>[4x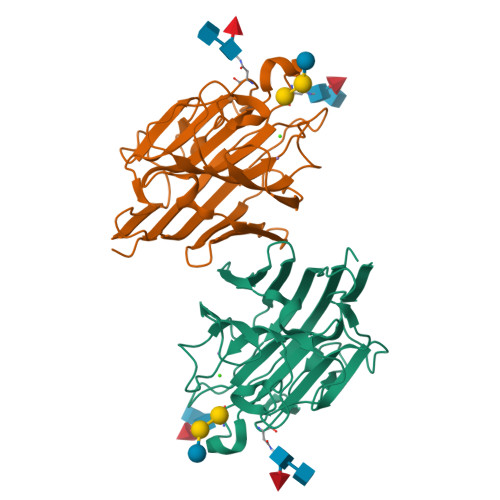]KTISFNFNQFHQNEEQLKLQRDARISSNSVLELTKVVNGVPTWNSTGRALYAKPVQVWDSTTGNVASFETRFSFSIRQPFPRPHPADGLVFFIAPPNTQTGEGGGYFGIYNPLSPYPFVAVEFDTFRNTWDPQIPHIGIDVNSVISTKTVPFTLDNGGIANVVIKYDASTKILHVVLVFPSLGTIYTIADIVDLKQVLPESVNVGFSAATGDPSGKQRNATETHDILSWSFSASLPG> MPEEK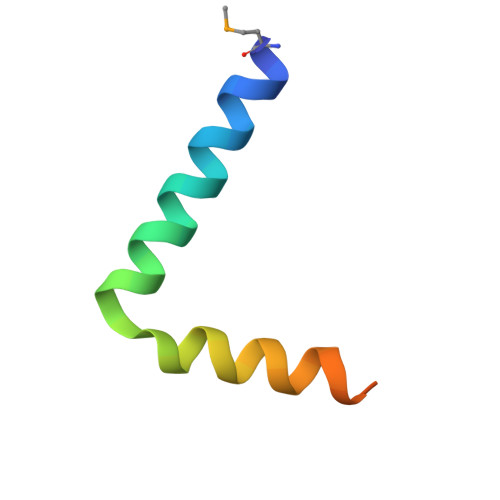ELLELLEELENIFSRSPSDIAEIVRLWFFERGLENLYF>GSHMVRESSFVEKMKKTGRNIIVFYGSQTGTAEEFANRLSKDAHRYGMRGMSADPEEYDLADLSSLPEIDNALVVFCMATYGEGDPTDNAQDFYDWLQETDVDLSGVKFAVFGLGNKTYEHFNAMGKYVD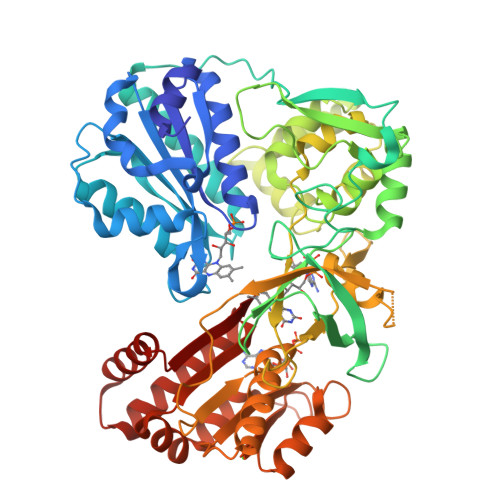KRLEQLGAQRIFELGLGDDDGNLEEDFITWREQFWLAVCEHFGVEATGEESSIRQYELVVHTDIDAAKVYMGEMGRLKSYENQKPPFDAKNPFLAAVTTNRKLNQGTERHLMHLELDISDSKIRYESGDHVAVYPANDSALVNQLGKILGADLDVVMSLNNLDEESNKKHPFPCPTSYRTALTYYLDITNPPRTNVLYELAQYASEPSEQELLRKMASSSGEGKELYLSWVVEARRHILAILQDCPSLRPPIDHLCELLPRLQARYYSIASSSKVHPNSVHICAVVVEYETKAGRINKGEATNWLRAKEPVGENGGRALVPMFVRKSQFRLPFKATTPVIMVGPGTGVAPFIGFIQERAWLRQQGKEVGETLLYYGCRRSDEDYLYREELAQFHRDGALTQLNVAFSREQSHKVYVQHLLKQDREHLWKLIEGGAHIYVCGDARNMARDVQNTFYDIVAELGAMEHAQAVDYIKKLMTKGRYSLDVWS[2x]> SRCTHLENRDFVTGTQGTTRVTLVLELGGCVTITAEGKPSMDVWLDAIYQENPAKTREYCLHAKLSDTKVAARCPTMGPATLAEEHQGGTVCKRDQSDRGWGNHCGLFGKGSIVACVKAACEAKKKATGHVYDANKIVYTVKVEPHTGDYVAANETHSGRKTASFTVSSEKTILTMGEYGDVSLLCRVASGVDLAQTVILELDKTVEHLPTAWQVHRDWFNDLALPWKHEGAQNWNNAERLVEFGAPHAVKMDVYNLGDQTGVLLKALAGVPVAHIEGTKYHLKSGHVTCEVGLEKLKMKGLTYTMCDKTKFTWKRAPTDSGHDTVVMEVTFSGTKPCRIPVRAVAHGSPDVNVAMLITPNPTIENNGGGFIEMQLPPGDNII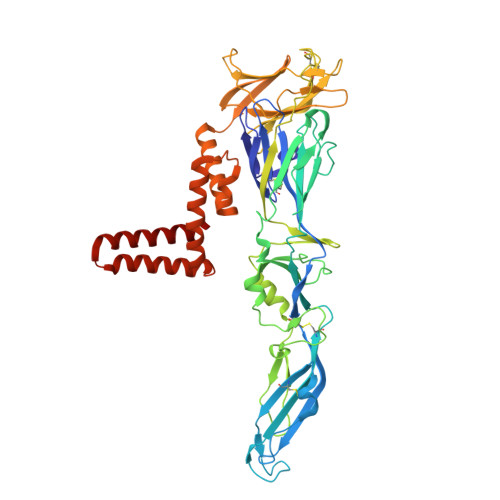YVGELSHQWFQKGSSIGRVFQKTKKGIERLTVIGEHAWDFGSAGGFLSSIGKAVHTVLGGAFNSIFGGVGFLPKLLLGVALAWLGLNMRNPTMSMSFLLAGGLVLAMTLGVGA>MGSSHHHHHHSSGLVPRGSHMPATHHSSATSAERPTVVGRIPVLDVRPVVQRGRRPAKAVTGESFEVSATVFREGHDAVGANVVLRDPRGRPGPWTPMRELAPGTDRWGATVTAGETGTWSYTVEAWGDPVTTWRHHARIKIPAGLDTDLVLEEGARLYERAAADVPGREDRRELLAAVDALRDESRPAASRLAAALTPQVDAVLARHPLRDLVTSSDPLPLLVERERALYGAWYEFFPRSEGTPHTPHGTFRTAARRLPAIAAMGFDVVYLPPIHPIGTTHRKGRNNTLSATGDDVGVPWAIGSPEGGHDSIHPALGTLDDFDHFVTEAGKLGLEIALDFALQCSPDHPWVHKHPEWFHHRPDGTIAHAENPPKKYQDIYPIAFDADPDGLATETVRILRHWMDHGVRIFRVANPHTKPVAFWERVIADINGTDPDVIFLAEAFTRPAMMATLAQIGFQQSYTYFTWRNTKQELTEYLTELSGEAASYMRPNFFANTPDILHAYLQHGGRPAFEVRAVLAATLSPTWGIYSG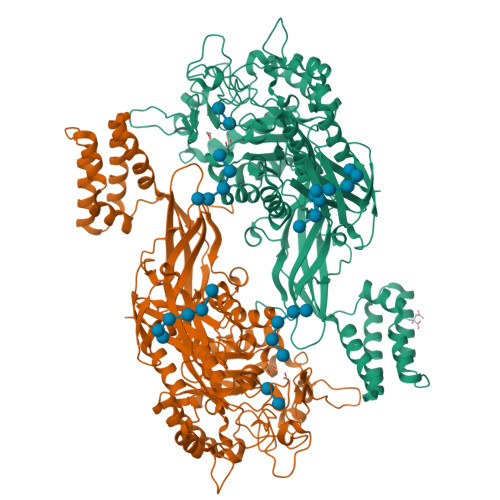YELCENTPLREGSEEYLDSEKYQLKPRDWTRAAREGTTIAPLVTRLNTIRRENPALRQLRDLHFHPTDKEEVIAYSKRQGSNTVLVVVNLDPRHTQEATVSLDMPQLGLDWHESVPVRDELTGETYHWGRANYVRLEPGRTPAHVCTVLRPSHPQIGGSHTT[2x]> VPMHPFVKALQEHFTAHQNPEKAEPMARYMKNHFLFLGI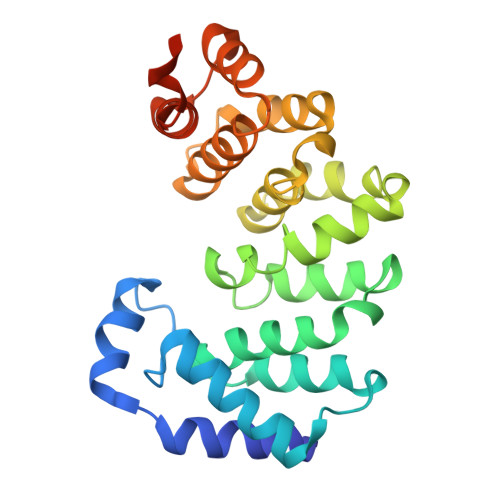QTPERRQLLKDIIQIHTLPDQKDFQIIIRELWDLPEREFQAAALDIMQKYKKHINETHIPFLEELIVTKSWWDSVDSIVPTFLGDIFLKHPELISAYIPKWIASDNIWLQRAAILFQLKYKQKMDEELLFWIIGQLHSSKEFFIQKAIGWVLREYAKTNPDVVWEYVQNNELAPLSKREAIKHIKQNYGINNEKIGETLS Cas12g is an endonuclease belonging to the type V RNA-guided CRISPR–Cas family. However, while most known type V effectors use this domain to cleave DNA substrates, Cas12g, the Cas effector of the newly identified type V-G systems, stands out by exhibiting RNA-guided ribonuclease (RNase) activity instead of cleaving DNA substrates. Cas12g, which is a thermostable protein identified from a hot spring metagenome locus, functions as an RNA-guided ribonuclease (RNase). Cas12g adopts a bilobed architecture encompassing recognition (REC) and nuclease (NUC) lobes.

The crystal structure of apo-Cas12g was determined at a resolution of 2.24 Å. We observed a single Cas12g in the asymmetric unit of the crystal structure. Apo-Cas12g exhibits a compact domain arrangement that differs from the extended conformations observed in apo-Cas12a. In the apo-Cas12g structure, two zinc finger motifs are located at the Helical 1 subdomain II, namely, the HCCC-type zinc finger (His248-Cys252-Cys323-Cys330) and the CCHC-type zinc finger (Cys228-Cys240-His335-Cys339). Each motif coordinates a Zn2+ ion and is referred to as Zn2+A (HCCC) and Zn2+B (CCHC) hereafter, respectively. Fortunately, the structure of apo-Cas12g determined in this study provides an intact view of the Helical 1 subdomain II, which consists of helices α9–α17. However, the density for the segment spanning aa 545–621 is absent, and only a helix can be observed in the Helical 2 domain. In addition, only three amino acids (aa 706–708) with visible density were detected in the Nuc domain, which is composed of 36 amino acids. In the inactive state of apo-Cas12g, the lid motif is positioned above the catalytic active site, obstructing the catalytic core region and preventing substrate binding and cleavage. In apo-Cas12g, the lid motif interacts with the Helical 1 subdomain II and Helical 2 domains and is held in place above the active site through hydrogen bonding between residues R661-R224, E666-R226 and K672-V632.

> MAQASSTPAVSPRPRPRYREERTLVRKLLPRPGQSKQEFRENVKKLRKAFLQFNADVSGVCQWAIQFRPRYGKPAEPTETFWKFFLEPETSLPPNDSRSPEFRRLQAFEAAAGINGAAALDDPAFTNELRDSILAVASRPKTKEAQRLFSRLKDYQPAHRMILAKVAAEWIESRYRRAHQNWERNYEEWKKEKQEWEQNHPELTPEIREAFNQIFQQLEVKEKRVRICPAARLLQNKDNCQYAGKNKHSVLCNQFNEFKKNHLQGKAIKFFYKDAEKYLRCGLQSLKPNVQGPFREDWNKYLRYMNLKEETLRGKNGGRLPHCKNLGQECEFNPHTALCKQYQQQLSSRPDLVQHDELYRKWRREYWREPRKPVFRYPSVKRHSIAKIFGENYFQADFKNSVVGLRLDSMPAGQYLEFAFAPWPRNYRPQPGETEISSVHLHFVGTRPRIGFRFRVPHKRSRFDCTQEELDELRSRTFPRKAQDQKFLEAARKRLLETFPGNAEQELRLLAVALGTDSARAAFFIGKTFQQAFPLKIVKIEKLYEQWPNQKQAGDRRDASSKQPRPGLSRDHVGRHLQKMRAQASEIAQKRQELTGTPAPETTTDQAAKKATLQPFDLRGLTVHTARMIRDWARLNARQIIQLAEENQVDLIVLESLRGFRPPGYENLDQEKKRRVAFFAHGRIRRKVTEKAVERGMRVVTVPYLASSKVCAECRKKQKDNKQWEKNKKRGLFKCEGCGSQAQVDENAARVLGRVFWGEIELPTAIPLEHHHHHH>[2x]G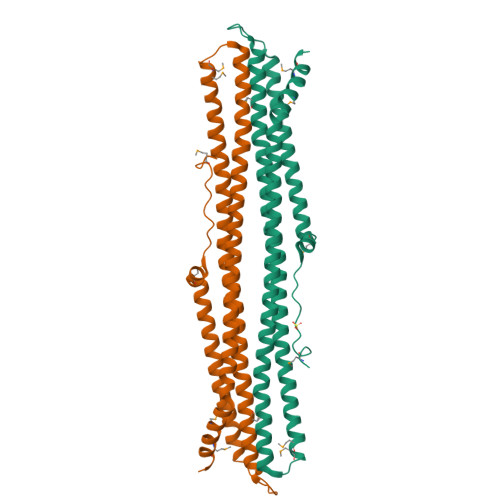AMDGNMKEVTQLPEPQTASLAELQQMKLFLKLLKKQEKELKELERKGSKRREELLQKYSVLFLEPVYPRGLDSQVVELKERLEMELIHLGEEYHDGIRRRKEQHATEQTAKITELAREKQIAELKALKESSESNIKDIKKKLEAKRLDRIQVMMRSTSDKAAQERLKKEINNSHIQEVVQTIKLLTEKTARYQQKLEEKQAENLRAIQEKEGQLQQEAVAEYEEKLKTLTVEVQEMVKNYMKEVFPDGPE>MSELIKENMHMKLYMEGTVNNHHFKCTSEGEGKPYEGTQTMKIKVVEGGPLPFAFDILATSFMYGSKTFINHTQGIPDFFKQSFP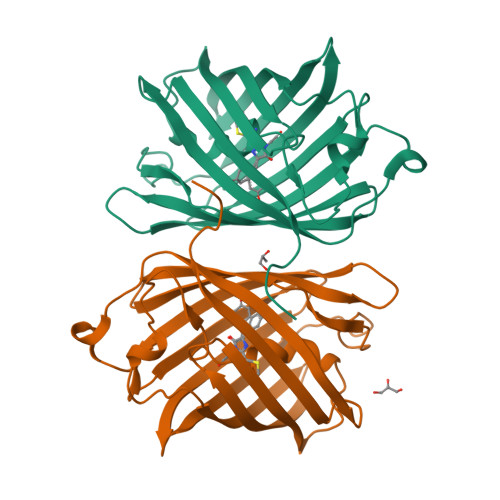EGFTWERITTYEDGGVLTATQDTSLQNGCIIYNVKINGVNFPSNGSVMQKKTLGWEANTEMLYPADGGLRGHSQMALKLVGGGYLHCSFKTTYRSKKPAKNLKMPGFHFVDHRLERIKEADKETYVEQHEMAVAKYCDLPSKLGHR[2x]>[12x]MSARR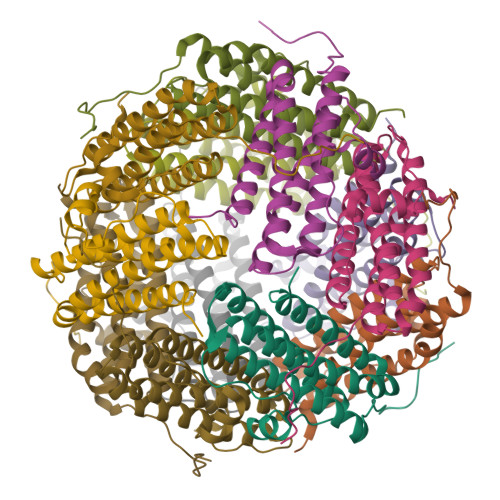TESDIQGFHATPEFGGNLQKVLVDLIELSLQGKQAHWNVVGSNFRDLHLQLDELVDFAREGSDTIAERMRALDAVPDGRSDTVAATTTLPEFPAFERSTADVVDLITTRINATVDTIRRVHDAVDAEDPSTADLLHGLIDGLEKQAWLIRSENRKV> MGPVWRKHYITYRINNYTPDMNREDVDYAIRKAFQVWSNVTPLKFSKINTGMADILVVFARGAHGDDHAFDGKGGILAHAFGPGSGIGGDAHFDEDEFWTTHSGGTNL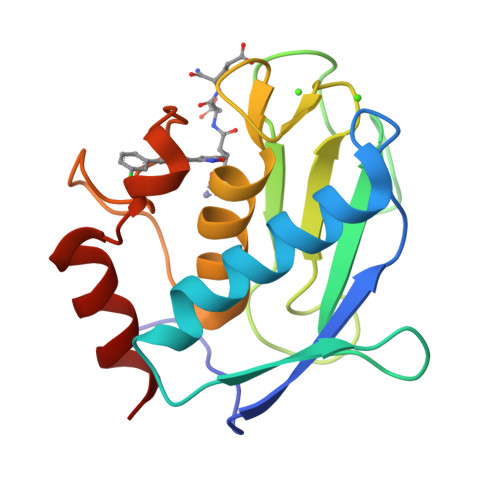FLTAVHEIGHSLGLGHSSDPKAVMFPTYAYVDINTFRLSADDIRGIQSLYG The protein TON_0340 (268 amino acids) was identified in a transcriptome study aimed at identifying genes whose expression is enhanced when this organism was grown with CO as the sole carbon and energy source. The biological function of TON_0340 is unknown, and a BLAST database search shows that TON_0340 belongs to the DUF4392 superfamily (after domain of unknown function), the members of which are found in all three domains of life. To gain insights into the biochemical function of TON_0340 and its homologues, we determined the crystal structures of TON_0340 in four different forms; the apo form without a bound metal ion and the Mn2+-, Mg2+- or Ca2+-bound form, revealing that the protein has a highly conserved bi-metal binding pocket. Our analyses strongly support that TON_0340 is a novel Mn2+-dependent phosphatase.

Intriguingly, in the crystals of the apo form of TON_0340, two protein molecules in the asymmetric unit also formed a dimer-like pair, but they were in parallel orientations. The intermolecular interactions are also mostly hydrophobic and bury a surface area of 1,778 Å2 in one subunit. The binding interface involves α2, α8 and α10, whereas that in the metal-bound TON_0340 involves α1, α2 and α10. The N-terminal segment corresponding to α1 in the metal-bound TON_0340 is disordered in both molecules forming the parallel dimer in the apo form. The helices α8 and α10 of one molecule interact withα8’ and α10’ of the other molecule, as if they form a four-helix bundle. Probably, the parallel dimer of TON_0340 is the biological unit in solution and the formation of the antiparallel dimer is likely to be caused by the high concentration of 2-methyl-2,4-pentanediol (16%) contained in the crystallization solution that probably disrupted the native hydrophobic interactions at the dimer interface. The apo-form of TON_0340 exhibited no detectable phosphatase activity.

>[2x]NRGVLKVYLDYRRKNFNFLHNSTKMFLDNLERVLIVTGFPIPPMMVAETDGPPGALAIYRAVEMLGGKAEILTYSEVEKALEPFGVSLARTPEPEDYSLIISVETPGRAADGRYYSMSALEIKRDPLDGIFLKARALGIPTIGVGDGGNEIGMGKIRELVVGHVPHGEKIASVVETDELIVSAVSNWGAYGLVAQASIEVGRNLLEGWDERRVIEAISSAGLIDGVSKTLAPSVDGIRLMVHEGIVELLKAVVDEAIKL>[2x]GSGFPIRLVDGENKK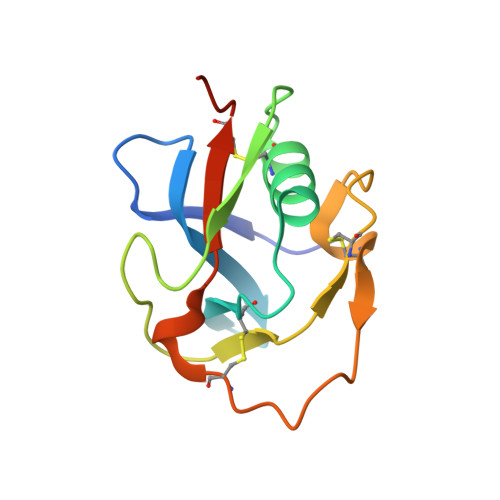EGRVEVFVNGQWGTICDDGWTDKHAAVICRQLGYKGPARARTMAYFGEGKGPIHMDNVKCTGNEKALADCVKQDIGRHNCRHSEDAGVICDYLEKKASS>HEMNSSKYVESPNYTKVEFGEHYARLRPKKLKANIEYTTPTGHIYRTDHKGRIKEVYVDNLSLKDGDRNSHAQRTVGGEDRLPDDDGGALIARMFGGSKDIDNLVAQSKFINRPFKEKGHWYNLEKEWQEFLNSGKEVKNIKMEVKYSGNSQRPTIFKVEYEINGERNIRRILNK[2x]

Toxin EsaD secreted by some S. aureus strains through the type VII secretion system (T7SS) specifically kills those strains lacking the antitoxin EsaG. EsaD is a toxin secreted in a T7SS machinery-dependent manner by S. aureus. Here we report the structures of EsaG, the nuclease domain of EsaD and their complex, which together reveal an inhibition mechanism that relies on significant conformational change of the toxin. The major contribution of this study is the discovery of an inhibitory mechanism in the toxin-antitoxin module that is based on a significant structural deformation of the toxin, where the central β-sheet of the nuclease domain of EsaD is split by EsaG into two fragments.

Due to cytotoxicity, the EsaD proteins used for crystallization were over-expressed in E. coli in an inactive state by mutating the catalytic H528 residue to Alanine (H528A). The crystal structures were determined at resolutions of 2.30 Å for the nuclease domain of EsaD (residues 440–614) and 2.60 Å for the EsaG-EsaD (residues 450–614, hereafter referred as EsaDc) complex, respectively. The nuclease domain of EsaD presents a typical fold of ββα-metal nucleases (also known as His-Me finger nucleases), even though they share low sequence similarity (<20%). The structure contains a central 6-stranded β-sheet that is largely open to solvent on one side and flanked by one short α-helix (αA) and the well-known ββα-metal finger motif on the other side. The ββα-metal finger (Residues 501–573), playing a critical role in nicking DNA, creates a compact catalytic center that is composed of two antiparallel β-strands (β4 and β5) connected by a long loop and linked to a C-terminal α-helix (αB). As observed in some other His-Me finger nucleases, αB is interrupted by a protruding ‘finger loop’ of unknown function. In addition, a long N-terminal loop (Residues 455–468) wraps around the central β-sheet from the β1 side and extends to the “back” face. Notice that the EsaG binding surface of the CFL part of the free EsaDc is exposed to the solvent, while that of the NFL part is buried and stabilized by the ββα-metal finger motif. There are two tryptophan residues in EsaDc (W560 and W567), both of which are buried in the free EsaDc structure, but exposed to solvent on the structure of the complex.> GPMTSQKLVRLPGLIDVHVHLREPGGTHKEDFASGTAAALAGGITMVCAMPNTRPPIIDAPALALAQKLAEAGARCDFALFLGASSENAGTLGTVAGSAAGLKLYLNETLSELRLDSVVQWMEHFETWPSHLPIVAHAEQQTVAAVLMVAQLTQRSVHICHVARKEEILLIKAAKARGLPV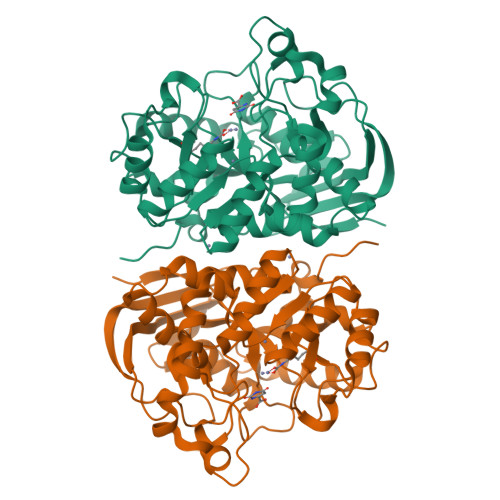TCEVAPHHLFLSHDDLERLGPGKGEVRPELGSRQDVEALWENMAVIDCFASDHAPHTLEEKCGSRPPPGFPGLETMLPLLLTAVSEGRLSLDDLLQRLHHNPRRIFHLPPQEDTYVEVDLEHEWTIPSHMPFSKAHWTPFEGQKVKGTVRRVVLRGEVAYIDGQVLVPPGYGQDVRKWPQGAVPQLPPSAPATSEMTTTPERPRRGIPGLPD>[2x]GSHNDKDLSTWQTFRRLWPTIAPFKAGLIVAGVALILNAASDTFMLSLLKPLLDDGFGKTDRSVLVWMPLVVIGLMILRGITSYVSSYCISWVSGKVVMTMRRRLFGHMMGMPVSFFDKQSTGTLLSRITYDSEQVASSSSGALITVVREGASIIGLFIMMFYYSWQLSIILIVLAPIVSIAIRVVSKRFRNISKNMQNTMGQVTTSAEQMLKGHKEVLIFGGQEVETKRFDKVSNRMRLQGMKMVSASSISDPIIQLIASLALAFVLYAASFPSVMDSLTAGTITVVFSSMIALMRPLKSLTNVNAQFQRGMAACQTLFTILDSEQEKDEGKRVIERATGDVEFRNVTFTYPGRDVPALRNINLKIPAGKTVALVGRSGSGKSTIASLITRFYDIDEGEILMDGHDLREYTLASLRNQVALVSQNVHLFNDTVANNIAYARTEQYSREQIEEAARMAYAMDFINKMDNGLDTVIGENGVLLSGGQRQRIAIARALLRDSPILILDEATSALDTESERAIQAALDELQKNRTSLVIAHRLSTIEKADEIVVVEDGVIVERGTHNDLLEHRGVYAQLHKMQFGQ

The ATP-binding cassette (ABC) transporter, MsbA, plays a pivotal role in lipopolysaccharide (LPS) biogenesis by facilitating the transport of the LPS precursor lipooligosaccharide (LOS) from the cytoplasmic to the periplasmic leaflet of the inner membrane. MsbA forms a homodimer and exhibits a topology similar to other ABC transporters, comprising two NBDs and two transmembrane domains (TMDs) containing 12 transmembrane helices. Upon binding ATP, MsbA undergoes dimerization of the NBDs, inducing rearrangement in the TMDs. An ATP hydrolysis-driven conformational change promotes the transition to an outward-facing (OF) conformation, facilitating the flipping of LOS to the periplasmic side of the inner membrane for further modifications.

The fifth MsbA structure adopts an open, outward-facing conformation and was resolved to a resolution of 2.7 Å. First, well-resolved density is observed for KDL binding, even for the six lipid tails. The positioning of KDL is centered on TM5, occupying a specific region within the cytoplasmic leaflet of the inner membrane. This location has recently been identified as the exterior LOS binding site of MsbA, a site that is important for stimulation of MsbA ATPase by hexaacylated lipid A species. The coordination of KDL is reminiscent of our recent structure with R188 and R238 interacting with the characteristic phosphoglucosamine (P-GlcN) moieties of LOS. However, an additional contact is formed between N235 and one of the Kdo molecules of the headgroup. While the structure is in an open, outward conformation, the transporter is not bound to nucleotide. The π–π interaction of Y351 of the A-loop with the adenosine moiety (observed in nucleotide bound structures) is substituted by a cation–π interaction with R354, priming the NBDs for binding ATP. Moreover, tube-like density is observed in the transmembrane region, in which we modeled the C10E5 detergent. The nucleotide-free open, outward facing conformation presented here suggests nucleotide is released post ATP hydrolysis prior to repopulating an IF conformation.> DLPPVAKAAQVVNQTLQLDDSYPDLDSYCRPGASSDYEMQSSDSSWAPFHVVRHHNIPDKVFEHLNAGEVFTKLGLFAEIGYAWASIDSSLFLWDYTHPNPELIGYEEATHTITAVALVPPKPGVFVKTITHVLVVATTSEIILLGVSATPTPSGSKSLTLYSTRMSVHRGGSDVSFIVGTKDGRIFLGGESDTDIHEIFYQQEERWFSSRCGKINHSHPFGSRQQEWLRGLYVDDTRNLLYSLSNRSTIRTYHMEGPEKLTKVIEKDKTSCLRDFAHMADSSPLFTDKTNIVALSPIPATEASKLHLMALTDTGCRLFLSATSSASYTMGGATALAPQSMQLQFVKFPPRESPTRIRTLNGQIIDSQLDKTSRALDPSALGFRFSPGYFFDVVR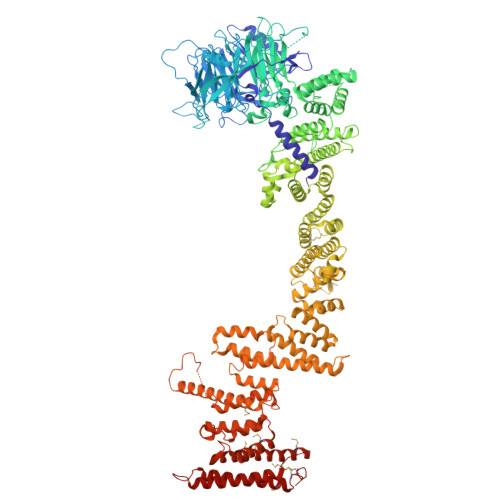KHPNQDMLFVSAPDTGRIKVTQPASALKYFEQGTWIELENGNRTIEIGLTTAPFAAAKQPLGFGNELAVQFDQVPGEFAVLTNTGVHIVRRRRLVDIFAKALGNCVSASDDALEREVRKFINQYGRVETIAAALAVACGQGSDLRTGTGRGMDRNTENLARAAFIEYGGQPRLAESDGKQSVSESVRLSSRHDALALYLTRLVRTLWKAKVVQVGSGSDISSTIPTSKLVTIQENVERLRNFLEANKSTIQGLAPPSERLFGRQEDIANQKEHQALHALQKLMESISEGISFVLMLFDERVSDIYARLDAVSQQQLKDLTYEQLFSQTPGKELAKVLVKAIVNRNIASGANVETVADALRRRCGSFCSPDDVVTFKAQEQLQRASEQAHNSPVLRALLAESLRLFEQVAGSLTPANLTTAVEQMISLKYYAGAIQLCLTVAQQKDRGNTALSWVNDGKPANDSRKKAFDERKICYNLIHQVLDKLESDFAGEPELVDGRPTLAATKRMEAYNVVNDSSDEVFHFDMYEWYIEKGWTDRILSIDSPHVITYLQRLAETDFRHAELLCRFYTTRSRFFEAAQVQTNLAKSDLNISLKDRIILLSRAKGNASVNTIGISRQQQQQLNHEASELLEIAHIQDDLLERLVADPRIPEERKAEIEEFLDGPIRTLTDLFNDYADQANYYDLCLLIFHAADFHNPRTIMDTWNNLINQSHFEAEQRREYWEIVQAGGDLPAGVIAPIAEPPLPYVYVSQQIQLIAHRTSLDSLIFPVNSLLPVVCAYAINNGQDASIGADPCWPIQLFLNLGVPHALMVQVLENVLDTQEAPFTGRRRKLVVQWIAMAVDMWVREVERRGAMAAAAASGASGSEAVMGSWVSELLGRADQVLTQIAGTGATLRGGAASDAEEIASLRRTVKGLKRSVDMLLGGEMARMSFFR However, intestinal bacterial GUSs cleave the attached glucuronic acid for use as a carbon source, allowing potentially toxic compounds to re-enter the enterohepatic circulation. However, microflora-encoding β-glucuronidases (GUSs) are notorious for reversing the glucuronidation to release SN-38 in the intestinal lumen and thus represent the major cause of undesirable effects. GUS contains a deep enzyme active site (the two catalytic glutamates lie ~12 Å below the protein surface). To understand the underlying structural basis, we prepared C6-propyl, -hexyl, and -nonyl UIFGs (2–4, respectively) and resolved the eight X-ray crystal structures of 1–4 bound to EcGUS or Bifidobacterium dentium GUS (BdGUS).

Uronic isofagomine (UIFG, 1) potently inhibits both mammalian and bacterial GUSs, owing to ionic interactions between the protonated ring nitrogen and the two catalytic glutamates. Inhibitor 1 appeared to be potent for both human and bacterial GUSs (e.g., Ki = 180 nM for HsGUS, 16 nM for EcGUS, 7.4 nM for BdGUS, 6.5 nM for CpGUS). Isothermal titration calorimetry was used to measure the thermodynamics of the binding of 1 or 2 to EcGUS and BdGUS. The potent inhibition of 1 was contributed mainly by enthalpy (ΔH = –10.47 and –9.12 kcal mol−1 for BdGUS and EcGUS, respectively).

>HMLRPVETPTREIKKLDGLWAFSLDRENCGIDQRWWESALQESRAIAVPGSFNDQFADADIRNYAGNVWYQREVFIPKGWAGQRIVLRFDAVTHYGKVWVNNQEVMEHQGGYTPFEADVTPYVIAGKSVRITVCVNNELNWQTIPPGMVITDENGKKKQSYFHDFFNYAGIHRSVMLYTTPNTWVDDITVVTHVAQDCNHASVDWQVVANGDVSVELRDADQQVVATGQGTSGTLQVVNPHLWQPGEGYLYELCVTAKSQTECDIYPLRVGIRSVAVKGEQFLINHKPFYFTGFGRHEDADLRGKGFDNVLMVHDHALMDWIGANSYRTSHYPYAEEMLDWADEHGIVVIDETAAVGFNLSLGIGFEAGNKPKELYSEEAVNGETQQAHLQAIKELIARDKNHPSVVMWSIANEPDTRPQGAREYFAPLAEATRKLDPTRPITCVNVMFCDAHTDTISDLFDVLCLNRYYGWYVQSGDLETAEKVLEKELLAWQEKLHQPIIITEYGVDTLAGLHSMYTDMWSEEYQCAWLDMYHRVFDRVSAVVGEQVWNFADFATSQGILRVGGNKKGIFTRDRKPKSAAFLLQKRWTGMNFGEKPQQGGKQ[4x]>MTKVLVLGGRFGALTAAYTLKRLVGSKADVKVINKSRFSYFRPALPHVAIGVRDVDELKVDLSEALPEKGIQFQEGTVEKIDAKSSMVYYTKPDGSMAEEEYDYVIVGIGAHLATELVKGWDKYGYSVCEPEFATKLREKLESFQGGNIAIGSGPFYQGHNPKP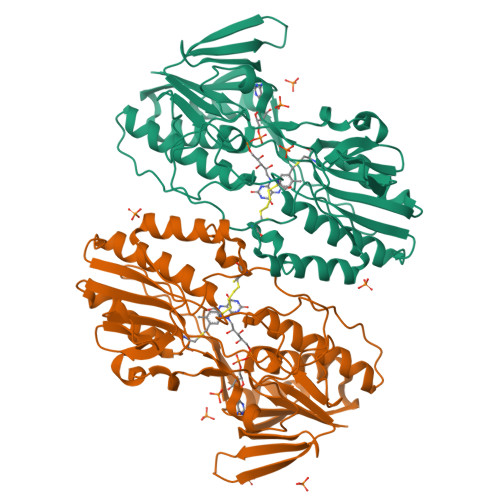KVPENFVPNADSACEGPVFEMSLMLHGYFKKKGMLDKVHVTVFSPGEYLSDLSPNSRKAVASIYNQLGIKLVHNFKIKEIREHEIVDEKGNTIPADITILLPPYTGNPALKNSTPDLVDDGGFIPTDLNMVSIKYDNVYAVGDANSMTVPKLGYLAVMTGRIAAQHLANRLGVPTKVDKYYPTIVCVADNPYEGYAVSVKDDTWYGGTVSIADPAAVNHLKKELFTKYYMWTKGDMALEKFLASW[2x]>GPMLADLDHFGKNYKHDEEAQRNQKPWMLTWPQIKLVLLAGVGFFLDAYDLFIINQVAPMLAQVYFPKTGLPAQRQDLMKAAANIGCVVGQVMFGVLGDSFGRKFVYGKELILIIVATIFQMSAPSHW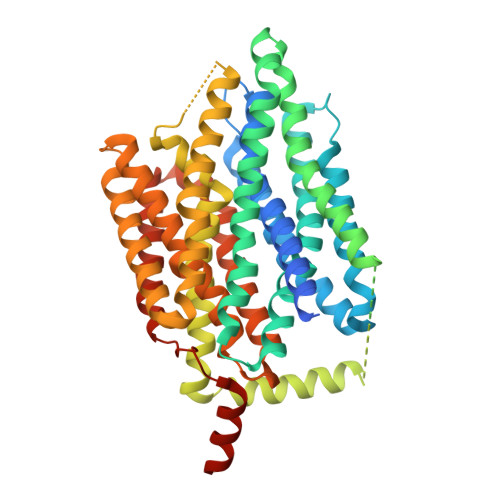DGNRVLTWITICRVFLGIGIGGDYPMSATVVSDRANIHRRGTLLCFIFANQGWGSFVGSLVTIVTISGFKHRLKSGHTHDVDKAWRILIGLSLIPAFGTLYQRLTLPESRKFELTRDAASSSTVAIDKKDHDATHEVKDAPESEKSSPKVTPADAIDDDRHGVIASKKAHWQEFVAYFSTWNHFRNLLGSMLGWFLVEIAFYGINLNQSVVLAQIGFAGKTGDVYDKLFQLATGNIIVTALGFLPGYYFTLFLIDIVGRKKLQFMGFIMSGLFLAILAGEIDHIGKGPLLACFTFMQFFFNFGANTTTFIVAAELFPTRIRASAHGISAAAGKCGAILSSLVFNQLKAKIGTSAVLWIFFSTCILGFISTFLIDETMGVDPDEKDLEERRARGEIPGGLVPR[2x]> NSIIGEKYRWPHTIPYVLEDSLEMNAKGVILNAFERYRLKTCIDFKPWAGETNYISVFKGSGCWSSVGNRRVGKQELSIGANCDRIATVQHEFLHALGFWHEQSRSDRDDYVRIMWDRILSGREHNFNTYSDDISDSLNVPYDYTSVMHYSKTAFQ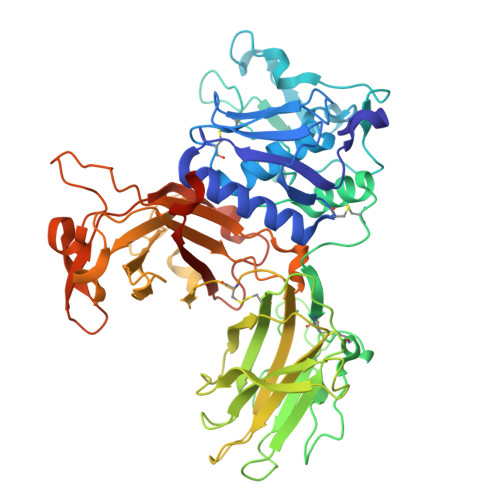NGTEPTIVTRISDFEDVIGQRMDFSDSDLLKLNQLYNCSSSLSFMDSCSFELENVCGMIQSSGDNADWQRVSQVPRGPESDHSNMGQCQGSGFFMHFDSSSVNVGATAVLESRTLYPKRGFQCLQFYLYNSGSESDQLNIYIREYSADNVDGNLTLVEEIKEIPTGSWQLYHVTLKVTKKFRVVFEGRKGSGASLGGLSIDDINLSETRCPHHIWHIRNFTQFIGSPNGTLYSPPFYSSKGYAFQIYLNLAHVTNAGIYFHLISGANDDQLQWPCPWQQATMTLLDQNPDIRQRMSNQRSITTDPFMTTDNGNYFWDRPSKVGTVALFSNGTQFRRGGGYGTSAFITHERLKSRDFIKGDDVYILLTVEDISHLNSTQIQLTPAPSVQDLCPSK> XXXXXXXXXXXXXXXXXXXXXXXXXXXXXXXXXXXXXXXXXXXXXXXXXXXXXXXXXXXXXXXXXXXXXXXXXXXXXXXXXXXXXXXXXXXXXXXXXXXXXXXXXXXXXXXXXXXXXXXXMALRDFCSVDGSDLFWEWNVTWNTSNPDFTKCFQNTVLVWVPCSYLWVCFPFYFLYLSHHDRGYIQMTHLNKAKTALGFLLWIVCWADLFYSFWERSMGKLLAPVFLVSPTLLGITMLLATFLIQIERRRGVQSSGIMLTFWLIALLCALAILRSKIMTALKEDARVDVFRDVTFYIYFSLVLIQLVLSCFSDRSPLFSETINDPNPCPESSASFLSRITFWWITGMMVQGYRQPLESTDLWSLNKEDTSEQVVPVLVKNWKKECAKSRKQPVKIVYSSKDPAKPKGSSKVDVNEEAEALIVKCPQKERDPSLFKVLYKTFGPYFLMSFLFKAVHDLMMFAGPEILKLLINFVNDKKAPEWQGYFYTALLFISACLQTLVLHQYFHICFVSGMRIKTAVIGAVYRKALVITNAARKSSTVGEIVNLMSVDAQRFMDLATYINMIWSAPLQVILALYLLWLNLGPSVLAGVAVMVLMVPLNAVMAMKTKTYQVAHMKSKDNRIKLMNEILNGIKVLKLYAWELAFKDKVLAIRQEELKVLKKSAYLAAVGTFTWVCTPFLVALSTFAVYVTVDENNILDAQKAFVSLALFNILRFPLNILPMVISSIVQASVSLKRLRVFLSHEDLDPDSIQRRPIKDAGATNSITVKNATFTWARNDPPTLHGITFSVPEGSLVAVVGQVGCGKSSLLSALLAEMDKVEGHVTVKGSVAYVPQQAWIQNISLRENILFGRQLQERYYKAVVEACALLPDLEILPSGDRTEIGEKGVNLSGGQKQRVSLARAVYCDSDVYLLDDPLSAVDAHVGKHIFENVIGPKGLLKNKTRLLVTHAISYLPQMDVIIVMSGGKISEMGSYQELLARDGAFAEFLRTYASAEQEQGQPEDGLAGVGGPGKEVKQMENGMLVTDTAGKQMQRQLSSSSSYSRDVSQHHTSTAELRKPGPTEETWKLVEADKAQTGQVKLSVYWDYMKAIGLFISFLSIFLFLCNHVASLVSNYWLSLWTDDPIVNGTQEHTQVRLSVYGALGISQGITVFGYSMAVSIGGIFASRRLHLDLLHNVLRSPISFFERTPSGNLVNRFSKELDTVDSMIPQVIKMFMGSLFNVIGACIIILLATPMAAVIIPPLGLIYFFVQRFYVASSRQLKRLESVSRSPVYSHFNETLLGVSVIRAFEEQERFIRQSDLKVDENQKAYYPSIVANRWLAVRLECVGNCIVLFASLFAVISRHSLSAGLVGLSVSYSLQVTTYLNWLVRMSSEMETNIVAVERLKEYSETEKEAPWQIQDMAPPKDWPQVGRVEFRDYGLR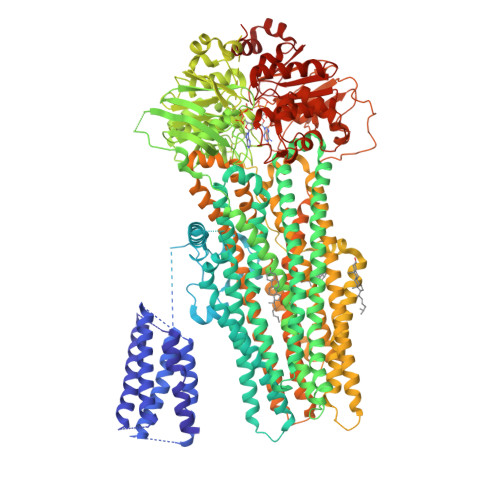YREDLDLVLKHINVTIDGGEKVGIVGRTGAGKSSLTLGLFRIKESAEGEIIIDDINIAKIGLHDLRFKITIIPQDPVLFSGSLRMNLDPFSQYSDEEVWTSLELAHLKGFVSALPDKLNHECAEGGENLSVGQRQLVCLARALLRKTKILVLDQATAAVDLETDDLIQSTIRTQFDDCTVLTIAHRLNTIMDYTRVIVLDKGEIQEWGSPSDLLQQRGLFYSMAKDSGLVSNSLEVLFQ>MSKTQEFRPLTLPPKLSLSDFNEFIQDIIRIVGSENVEVISSKDQIVDGSYMKPTHTHDPHHVMDQDYFLASAIVAPRNVADVQSIVGLANKFSFPLWPISIGRNSGYGGAAPRVSGSVVLDMGKNMNRVLEVNVEGAYCVVEPGVTYHDLHNYLEANNLRDKLWLDVPDLGGGSVLGNAVERGVGYTPYGDHWMMHSGMEVVLANGELLRTGMGALPDPKRPETMGLKPEDQPWSKIAHLFPYGFGPYIDGLFSQSNMGIVTKIGIWLMPNPGGYQSYLITLPKDG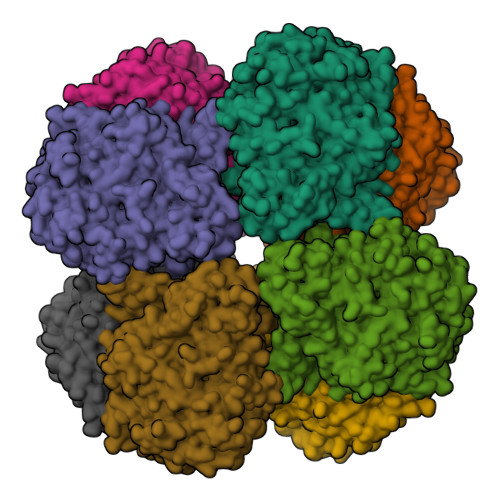DLKQAVDIIRPLRLGMALQNVPTIRHILLDAAVLGDKRSYSSRTEPLSDEELDKIAKQLNLGRWNFYGALYGPEPIRRVLWETIKDAFSAIPGVKFYFPEDTPENSVLRVRDKTMQGIPTYDELKWIDWLPNGAALFFSPIAKVSGEDAMMQYAVTKKRCQEAGLDFIGTFTVGMREMHHIVCIVFNKKDLIQKRKVQWLMRTLIDDCAANGWGEYRTHLAFMDQIMETYNWNNSSFLRFNEVLKNAVDPNGIIAPGKSGVWPSQYSHVTWKL[2x]>QTKKAAIVELLKQLELGLVPYDDIKQLIRRELARRLQWGYKPTYEEQIAEIQNLTHSLRQMKIATEVETLDSQLYEIPIEFLKIMNGSNLKGSCCYFKEDSTTLDEAEIAMLDLYCERAQIQDGQSVLDLGCGQGALTLHVAQKYKNCRVTAVTNSVSQKEYIEEESRRRNLLNVEVKLADITTHEMAETYDRILVIELFEHMKNYELLLRKISEWISKDGLLFLEHICHKTFAYHYEPLDDDDWFTEYVFPAGTMIIPSASFFLYFQDDVSVVNHWTLSGKHFSRTNEEW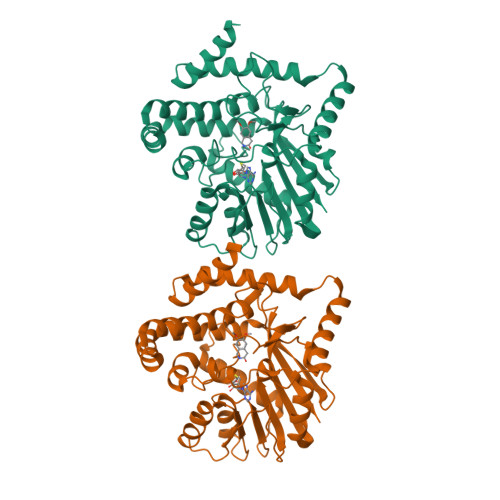LKRLDANLDVIKPMFETLMGNEEEAVKLINYWRGFCLSGMEMFGYNNGEEWMASHVLFKK[2x]> AYSTREILLALCIRDSRVHGNGTLHPVLELAARETPLRLSP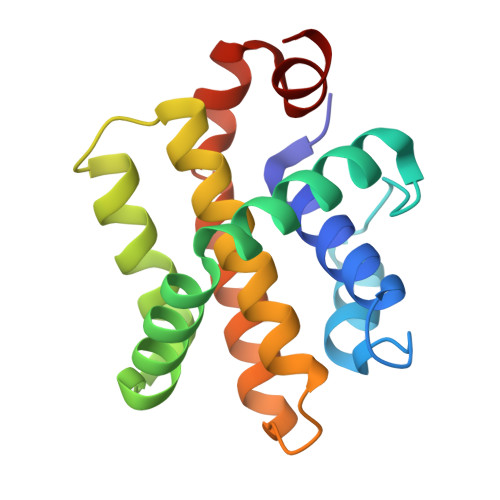EDTVVLRYHVLLEEIIERNSETFTETWNRFITHTEHVDLDFNSVFLEIFHRGDPSLGRALAWMAWCMHACRTLCCNQSTPYYVVDLSVRGMLEASEGLDGWIHQQGGWSTLIEDN>MSKWTYFGPDGENSWSKKYPSCGGLLQSPIDLHSDILQYDASLTPLEFQGYNLSANKQFLLTNNGHSVKLNLPSDMHIQGLQSRYSATQLHLHWGNPNDPHGSEHTVSGQHFAAELHIVHYNSDLYPDASTASNKSEGLAVLAVLIEMGSFNPSYDKIFSHLQHVKYKGQEAFVPGFNIEELLPERTAEYYRYRGSLTTPPCNPTVLWTVFRNPVQISQEQLLALETALYCTHMDDPSPREMINNFRQVQKFDERLVYTSFSQ[4x]

The carbonic anhydrase (CA) family (CA, EC 4.2.1.1), consisting of twelve catalytically active human isozymes, performs the catalysis of reversible hydration of CO2 into bicarbonate and acid protons. Since it has been observed that CAIX isozyme is highly overexpressed in numerous cancers, it has been postulated that compounds inhibiting CAIX may possess the anticancer activity and may be used in tumor treatment. Here we have designed a series of compounds, methyl 5-sulfamoyl-benzoates, which bear a primary sulfonamide group, a well-known marker of CA inhibitors, and determined their affinities for all twelve CA isozymes. Eight crystal structures of CA complexes with compounds are presented in this study: 9a bound to CAI and CAII, 3b, 3d, 5b, and 9a bound to CAXII, 3b bound to CAIX and mimic-CAIX (mutant of CAII containing amino acids in the active site as in CAIX: A65S, N67Q, I91L, F130V, V134L, and L203A).

Compound 9a was found at an identical position in the active sites of CAII and CAXII. The same binding mode of 9a in CAII and CAXII could be explained by the same interactions between the compound and conservative residues of these active sites. On the other hand, the binding affinity for CAXII differed from CAII by a factor of 26 (Kd_intr = 0.020 nM or ΔGintr = −63.1 kJ/mol for CAII vs. Kd_intr = 0.51 nM or ΔGintr = −55.2 kJ/mol for CAXII). For this reason, the binding of this compound to CAII was 26-fold stronger than for CAXII. Like the previous pair, these compounds differ only by their meta- groups: compound EA3-2o contains -NH(CH2)2OH, while 9a contains -OCH3. The positions of both compounds were not similar in CAXII; the para-benzene rings had slightly different orientations, and they were directed into the center of the active site cavity. Their orientation was defined by the bulky SO2 group of the linker, which was in contact with the protein surface. The EA3-2o bound to CAXII with 3.4-fold greater affinity than 9a (Kd_intr = 0.12 nM, ΔGintr = −59.0 kJ/mol vs. Kd_intr = 0.51 nM ΔGintr = −55.2 kJ/mol).> AQ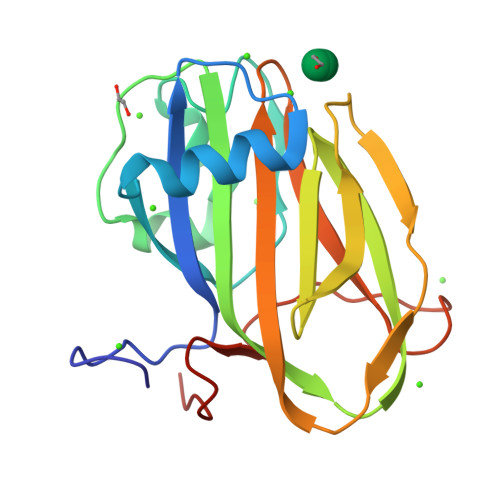DDSTPDSLFAGLVGEYYGTNSQLNNISDFRALVDSKEADATFEAANISYGRGSSDVAKGTHLQEFLGSDASTLSTDPGDNTDGGIYLQGYVYLEAGTYNFKVTADDGYEITINGNPVATVDNNQSVYTVTHASFTISESGYQAIDMIWWDQGGDYVFQPTLSADGGSTYFVLDSAILSSTGETPYTTA> GAACGACAGAG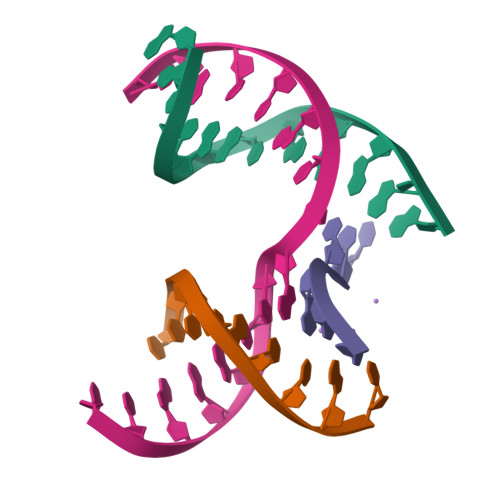A;> CGCCGACTC;> TCTGCG;> TCGAGTCGCTGTCGT>SNAQFGGLPVPLDQTLPLNVNPALPLSPTGLAGSLTNALSNGLLSGGLLGIMENLPLLDILKPGGGTSGGLLGGLLGKVTSVIPGLNNVIDIKVTDPQLLELGLVQSPDGHRLYVTIPLGIKLQVNTPLVGASLLRLAVKMDITAEILAVRDKQERIHLVLGDCTHSPGSLQISLLDGLGPLPIQGLLDSLTGILNKVLPELVQGNVCPLVNEVLRGLDITLVHDIVNML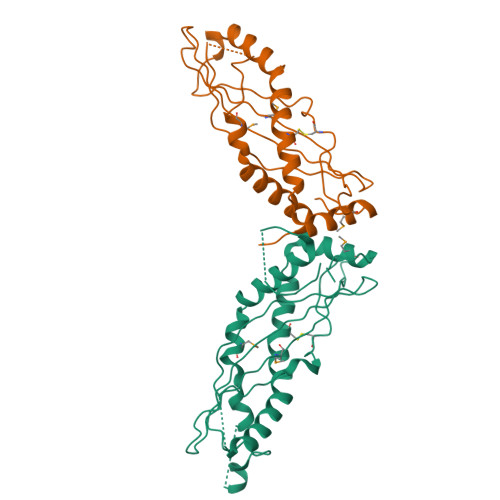IHGLQFVIKV[2x]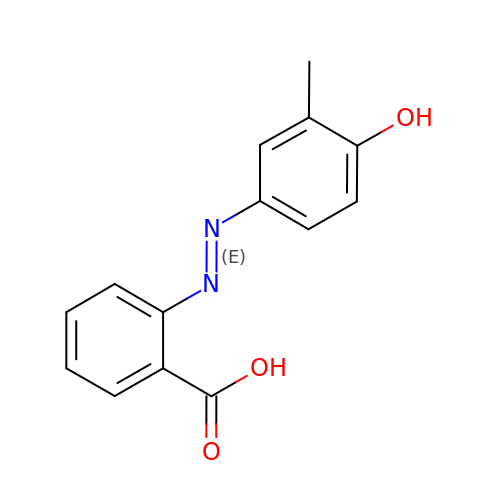2-((3'-METHYL-4'-HYDROXYPHENYL)AZO)BENZOIC ACID | C14 H12 N2 O3 | SBSCJWJICRGLIV-FOCLMDBBSA-N>[2x]GPLGSPILELKEKIQPEILELIKQQRLNRL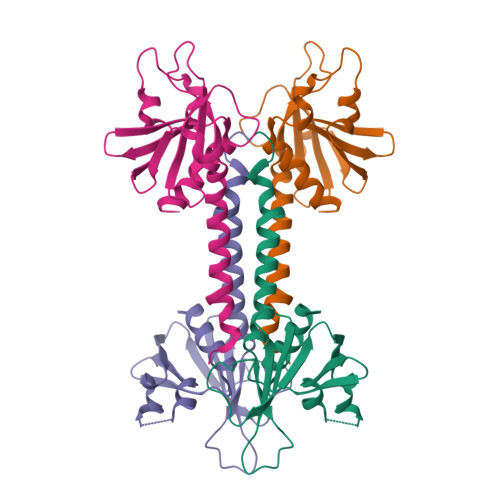VEGTCFRKLNARRRQDKFWYCRLSPNHKVLHYGDLEESPQGEVPHDSLQDKLPVADIKAVVTGKDCPHMKEKGALKQNKEVLELAFSILYDSNCQLNFIAPDKHEYCIWTDGLNALLGK> MSLQLLRNTRIFVSTVKTGHDTTNTQEILVQDDISWGQDSNSTDITVNEAGPRPTRGSKRFNDSLNAAEWSFSTYILPYEDTTTGKQIVPDYMLWHALSSGKAIDLDGDTGAHNNATNFMVNFKDNAYHELAMLHIYILTDNAWSYIDSCQINQAEVNVDIEDIGRVTWSGNGNQLIPLDEQPFDPDALGIDDETYMTIQSSYIKNKLTILKIKDMDSDKEYDIPITGGTFTINNNITYLTPNIMSRVNIPIGSFTGAFELTGSLTAYLNDKSLGSMELYKDLVRTLKVVNRFEIALILGGEYDDERPAAVLVAKQAHVNIPTIETDDVLGTSVEFKAIPTDLDTGDEGYLGFSNKYTKTTVANLIATGDGAETPPILVESITVKSAADATSVTNSDTLQMSVEVTPPEATNTAVTWSISSGDAATIDAESGLLTADVSKTGEVIVKAVAKDGSGVEGTKTITVSAGE

The T5 family of viruses are tailed bacteriophages characterized by a long non-contractile tail. The bacteriophage DT57C is closely related to the paradigmal T5 phage, though it recognizes a different receptor (BtuB) and features highly divergent lateral tail fibers (LTF). We present a composite map determined by electron cryo-microscopy (cryo-EM) at resolutions ranging between 2.9 Å to 4.9 Å of the entire T5-like phage particle DT57C, and atomic models comprising its core structural proteins. Our results provide a complete atomic structure of a T5-like phage, provide insights into the process of DNA ejection as well as a structural basis for the design of engineered phages and future mechanistic studies.

The tail of DT57C is composed of 40 stacked rings of tail tube protein (TTP), with each ring containing three subunits. The tail has helical symmetry and 3-fold rotational symmetry, with a rise 41.8 Å and twist 39.5°. While the local resolution of our reconstruction at the flexible Ig-like domains was too low for de novo model building, a predicted structure fitted the molecular envelope well. The tail shaft structure of DT57C is nearly identical to a previously published T5 tail tube structure. To better address tail flexibility and curvature of the segments, we performed asymmetrical reconstruction without imposition of any symmetry, which clearly revealed the presence of TMP inside the tail. Thus, the overall TMP organization within the tail tube of the phage DT57C can be described as a three-stranded parallel coiled coil, with α-helical secondary structure at least at its N- and C-termini (in accordance with secondary structure prediction).(2E)-4-amino-3-methylbut-2-en-1-yl 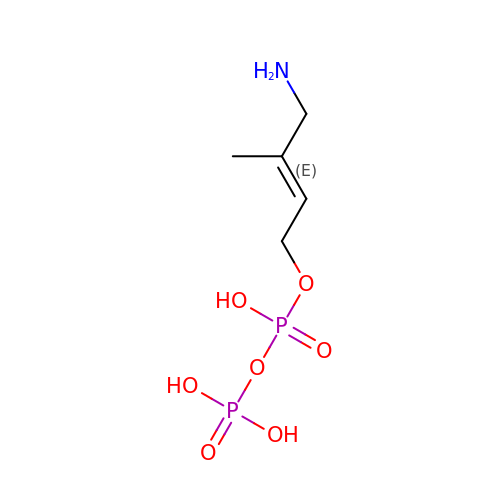trihydrogen diphosphate | C5 H13 N O7 P2 | SZAMOALLMIAULD-GORDUTHDSA-N> MAQQRALPQSKETLLQSYNKRLKDDIKSIMDNFTEIIKTAKIEDETQVSRATQGEQDNYEMHVRAANIVRAGESLMKLVSDLKQFLILNDFPSVNEAIDQRNQQLRTLQEECDRKLITLRDEISIDLYELEEEYYSSS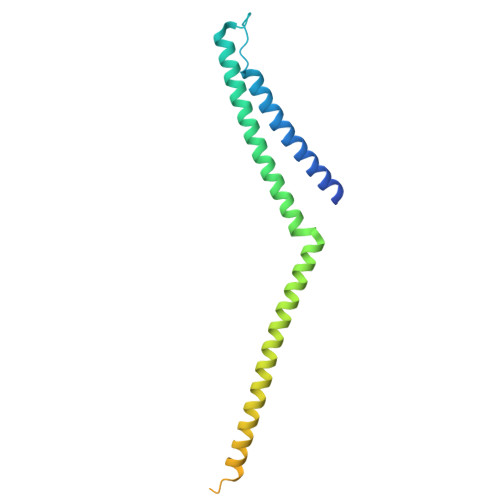SSLCEANDLPLCEAYGRLDLDTDSADGLSAPLLASPEPSAGPLQVAAPAHSHAGGPGPTEHA> HMKTVLMVAEKPSLAQSIAKILSRGSLSSHKGLNGACSVHEYTGTFAGQPVRFKMTSVCGHVMTLDFLGKYNKWDKVDPAELFSQAPTEKKEANPKLNMVKFLQVEGRGCDYIVLWLDCDKEGENICFEVLDAVLPVMNKAHGGEKTVFRARFSSITDTDICNAMACLGEPDHNEALSVDARQELDLRIGCAFTRFQTKYFQGKYGDLDSSLISFGPCQTPTLGFCVERHDKIQSFKPETYWVLQAKVNTDKDRSLLLDWDRVRVFDREIAQMFLN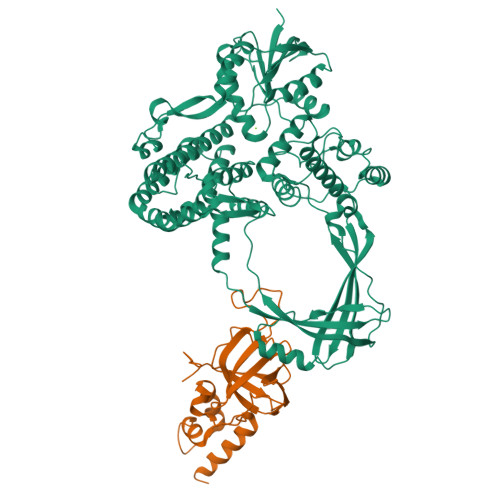MTKLEKEAQVEATSRKEKAKQRPLALNTVEMLRVASSSLGMGPQHAMQTAERLYTQGYISYPRTETTHYPENFDLKGSLRQQANHPYWADTVKRLLAEGINRPRKGHDAGDHPPITPMKSATEAELGGDAWRLYEYITRHFIATVSHDCKYLQSTISFRIGPELFTCSGKTVLSPGFTEVMPWQSVPLEESLPTCQRGDAFPVGEVKMLEKQTNPPDYLTEAELITLMEKHGIGTDASIPVHINNICQRNYVTVESGRRLKPTNLGIVLVHGYYKIDAELVLPTIRSAVEKQLNLIAQGKADYRQVLGHTLDVFKRKFHYFVDSIAGMDELMEVSFS;> GPGHMAQVAGAALSQAGWYLSDEGIEACTSSPDKVNVNDIILIALNTDLRTIGKKFLPSDINSGKVEKLEGPCVLQIQKIRNVAAPKDNEESQAAPRMLRLQMTDGHISCTAVEFSYMSKISLNTPPGTKVKLSGIVDIKNGFLLLNDSNTTVLGGEVEHLIEKW> MKLERVTVKNFRSHSDTVVEFKEGINLIIGQNGSGKSSLLDAILVGLYWPLRIKDIKKDEFTKVGARDTYIDL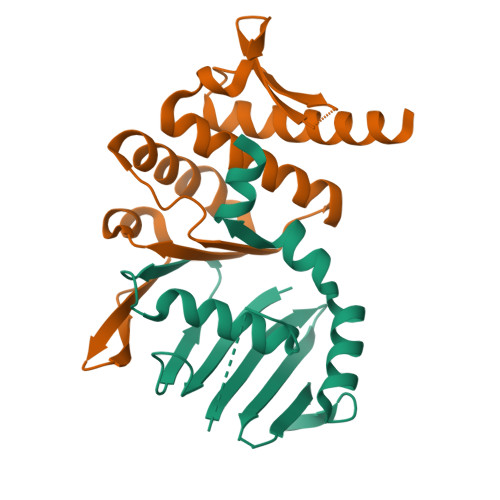IFEKDGTKYRITRRFLKGYSSGEIHAMKRLVGNEWKHVTEPSSKAISAFMEKLIPYNIFLNAIYIRQGQIDAIL;> LAREAALSKIGELASEIFAEFTEGKYSEVVVRAEENKVRLFVVWEGKERPLTFLRGGERIALGLAFRLAMSLYLAGEISLLILDEPTPYLDEERRRKLITIMERYLKKIPQVILVSHDEELKDAADHVIRISLENGSSKVEVVS>[2x]MHHHHHHHMAAQAAPAAAKAAAPSISRDEVEKCINAIRFLAIDAINKSKSGHPGMPMGCAPMGYVLWNEVMKYNPKNPDFFNRDRFVLSAGHGSMFQYSMMHLTGYDSVPLDQIKQFRQWNSLTPGHPENFVTPGVE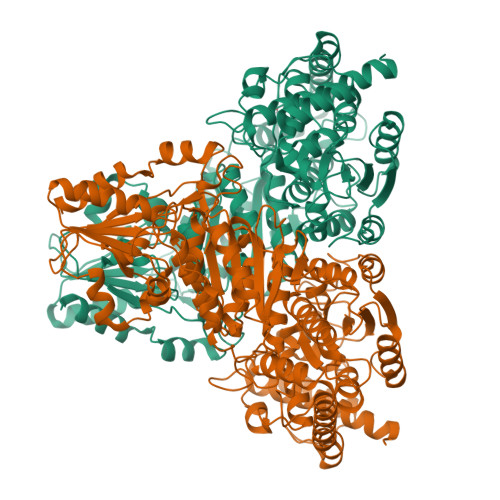VTTGPLGQGICNAVGLAVAEAHLAARFNKPDVKPIVDHYTYCILGDGCMMEGISNEACSLAGHWGLGKLIALYDDNKISIDGHTDISFTEDVAKRYEALGWHVIHVINGNTDVDGLRAAIAQAKAVKDKPTLIKVSTLIGYGSPNKADSHDVHGAPLGPDETAATRKNLNWPYGEFEVPQDVYDVFRGAIKRGAEEEANWHKACAEYKAKYPKEWAEFEALTSCKLPENWEAALPHFKPEDKGLATRQHSQTMINALAPALPGLIGGSADLAPSNLTLMKISGDFQKGSYAERNLRFGVREHAMGAICNGIALHKSGLIPYCATFYIFTDYMRNAMRMSALSEAGVVYVMTHDSIGLGEDGPTHQPIEHLASFRAMPDMLMIRPAGGNETAGAYKVAIANRKRPTTIALSRQNMPNIPNCSVEGVAKGAYTIHDTKAGVKPDVILMGTGSELELATAAAGILEKEGKNVRVVSFPCWELFEEQSAEYKESVLPSDVTARVSVEAATSFGWAKYIGLKGKHVGIDTFGASAPAPTLYEKFGITVNHVVEAAKATLQH> MFRNILSLVTKPSKLSQKTFYNFAAAKNEVQVSKKQQQAGAKRDLTQYVEGQIVNRNQLTLKKQEDIEQYVLKLVRGYFRTTNKQGLNINSVLQDHGLDEFDSIELAMQVEEDLGYVISAETIPVLNKVK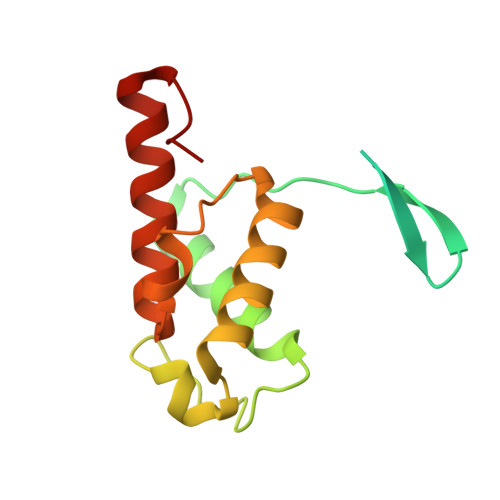HFVNYINHVEQFKAENGKAPIA> MKKAVINGEQIRSISDLHQTLKKE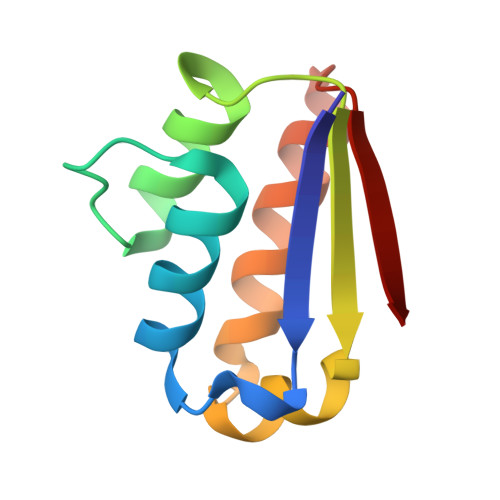LALPEYYGENLDALWDALTGWVEYPLVLEWRQFEQSKQLTENGAESVLQVFREAKAAGADITIILS> ATCDDGRTTANAACCILFPILDDIQENLFDG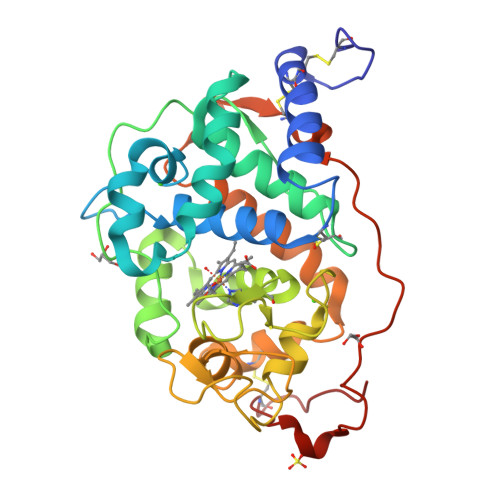AQCGEEVHESLRLTFHDAIGFSPTLGGGGADGSIIAFDTIETNFPANAGIDEIVSAQKPFVAKHNISAGDFIQFAGAVGVSNCPGGVRIPFFLGRPDAVAASPDHLVPEPFDSVDSILARMGDAGFSPVEVVWLLASHSIAAADGVDPSIPGTPFDSTPEVFDSQFFIETQLKGRLFPGTADNKGEAQSPLQGEIRLQSDHLLARDPQTACEWQSMVNNQPKIQNRFAATMSKMALLGQDKTKLIDCSDVIPTPPALVGAAHLPAGFSLSDVEQACAATPFPAL4-{[9-CHLORO-7-(2,6-DIFLUOROPHENYL)-5H-PYRIMIDO[5,4-D][2]BENZAZEPIN-2-YL]AMINO}BENZOIC ACID | C25 H15 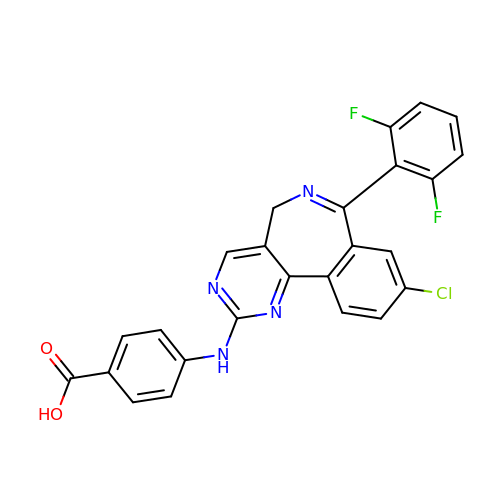Cl F2 N4 O2 | HHFBDROWDBDFBR-UHFFFAOYSA-N>GGEPAWDSPLRRVLAELNRIPSSRRRAARLFEWLIAPMPPDHFYRRLWEREAVLVRRQDHTYYQGLFSTADLDSMLRNEEVQFGQHLDAARYINGRRETLNPPGRALPAAAWSLYQAGCSLRLLCPQAFSTTVWQFLAVLQEQFGSMAGSNVYLTPPNSQGFAPHYDDIEAFVLQLEGRKLWRVYRPRVPTEELALTSSPNFSQDDLGEPVLQTVLEPGDLLYFPRGFIHQAECQDGVHSLHLTLSTYQRNTWGDFLEAILPLAVQAAMEENVEFRRGLPRDFMDYMGAQHSDSKDPRRTAFMEKVRVLVARLGHFAPVDAVADQRAKDFIHDSLPPVLTDRERALSVYGLPIRWEAGEPVNVGAQLTTETEVHMLQDGIARLVGEGGHLFLYYTVENSRVYHLEEPKCLEIYPQQADAMELLLGSYPEFVRVGDLPCDSVEDQLSLATTLYDKGLLLTKMPLALN[4x]

Nucleolar protein 66 (NO66) is a JmjC domain-containing protein which has been reported to be a histone demethylase and a ribosome protein 8 (Rpl8) hydroxylase. Nucleolar protein 66 (NO66) is a metazoan JmjC domain-containing protein that is highly conserved throughout evolution and was initially identified as a dual-location intranuclear protein. Evidence from a recent study indicated that NO66 hydroxylates ribosome protein 8 (Rpl8) and controls the biogenesis of the ribosome, which is consistent with the observation that NO66 is a constitutive nucleolar component. Moreover, previous work demonstrated that NO66 assembles as a tetramer and that the binding site of NO66 to osterix is located on the surface formed by a hinge region (interface I) from neighbouring subunits in the tetramer.

Our previous analyses demonstrated that NO66176–C exists as a tetramer in solution. We further compared the tetrameric structure of the NO66176–C–Ni2+ and NO66176–C–Rpl8204–224 complexes. In contrast to the similarity of the monomeric structure, the relative positions of the active sites of each subunit change in the two structures. The distance between the active sites in the dimer linked by interface II is 1.8 Å closer in the complex structure than in NO66176–C–Ni2+. When binding to substrate, the relative positions of each subunit in the NO66 tetramer shift. Oligomerization may facilitate the motion of each subunit in the NO66 tetramer and affect the catalytic activity.> SMQDPTIFEERHLKYISQLGKGNFGSVELCRYDPLGDNTGALVAVKQLQHSGPDQQRDFQREIQILKALHSDFIVKYRGVSYGPGRQSLRLVMEYLPSGCLRDFLQRHRARLDASRLLLYSSQICKGMEYLGSRRCVHRALAARNILVESEAHVKIADFGLAKLLPLDKDYYVVREPGQSPIFWYAPESLSDNIFSRQSDVWSFGVVLYELFTYCDKSCSPSAEFLRMM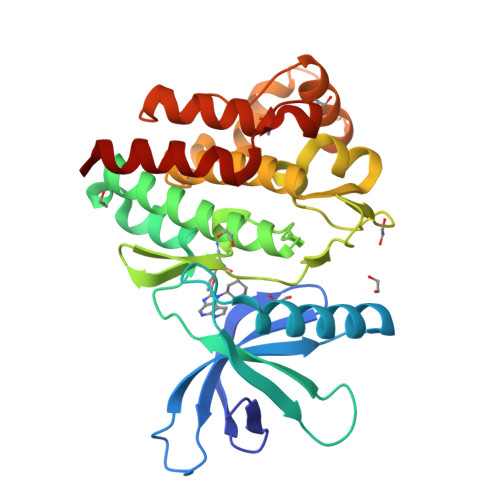GSERDVPALSRLLELLEEGQRLPAPPACPAEVHELMKLCWAPSPQDRPSFSALGPQLDMLWSGSR> MGSHHHHHHGSENLYFQSGSGSDENDTARKIIKTLLDIMREGDEDKLRDQMDPNVRADVGDKTVHGREHAA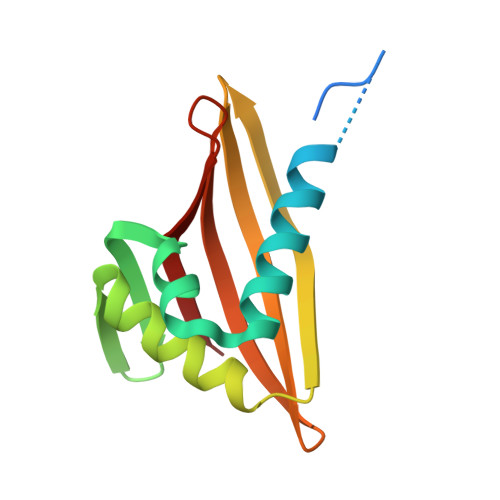KFLAHIVKRADHISITLKSLHNHNGRLRMQAEVRIVHNGRTERVTLEMVFRDHNGKLLIERMKYG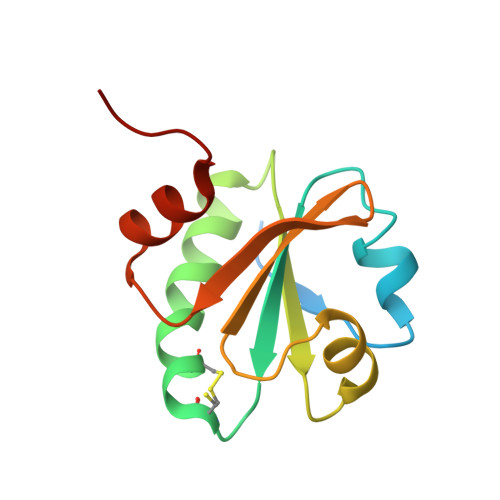> MAHHHHHHMTDAEKAIATIEVSDASFSTDVLASNKPVLVDFWATWCGPCKMVAPVLEEIASERGDHLTVAKLDVDANPETAQNFQVVSIPTLILFKDGQPVKRIVGAKGKAALLRELSDAVPNLG> MAAERLDPWGAVEIKDYDRLLRTFGIRPFSEVLPLLRKAGMEPSFLMRRGIIFGHRDFDKILEAKARGERVAVLTGFMPSGKFHFGHKLTVDQLIYLQKNGFKVFVAIADAEAFAVRRIGREEAVRIAVEEYIANMIALGLDPKDTEFYFQTNRGTPYFRLIQLFSGKVTAAEMEAIYGELTPAKMMASLTQAADILHVQLDEYGGYRHVVVPVGADQDPHLRLTRDLADRMAGVVELERPASTYHKLQPGLDGRKMSSSRPDSTIFLTDPPEVARNKLFRALTGGRATAEEQRRLGGVPEVCSVYHMDLYHLMPDDGEVKHIYT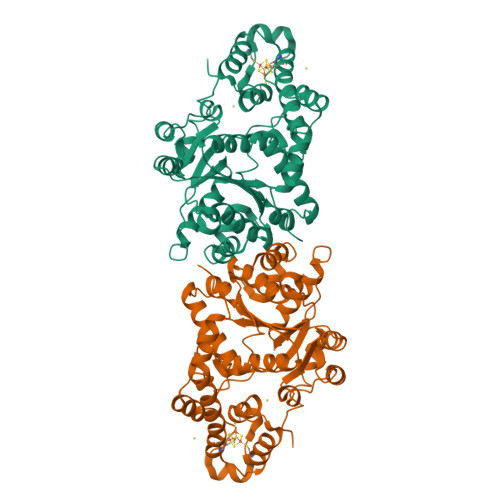SCRLGKILCGECKQIAWEKLERFLAEHQSRLEKAKTIAWKLVEPPRF>GGGVMHYTDKAALPADGEAREVAALFDTWNAALATGNPHKVADLYAPDGVLLPTVSNEVRASREQIENYFEMFLTKKPKGVIN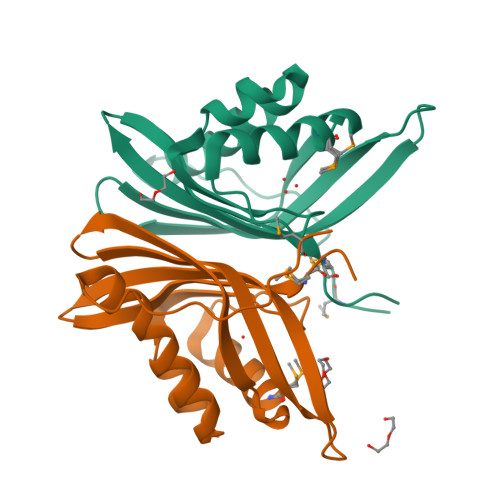YRTVRLLDDDSAVDAGVYTFTLTDKNGKKSDVQARYTFVYEKRDGKWLIINHHSSAMPEVDTATATAAVTKAK[2x]> PATRILLLVLAVIIYGTAGFHFIE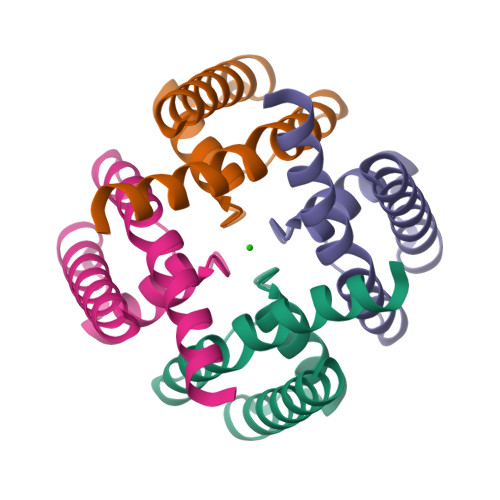GESWTVSLYWTFVTIATVGYGDYSPHTPLGMYFTCTLIVLGIGTFAVAVERLLEFLI> RGVEGSTKSIKYLLFVFNFVFWLAGGVILGVALWLRHDPQTTNLLYLELGDKPAPNTFYVGIYILIAVGAVMMFVGFLGCYGAI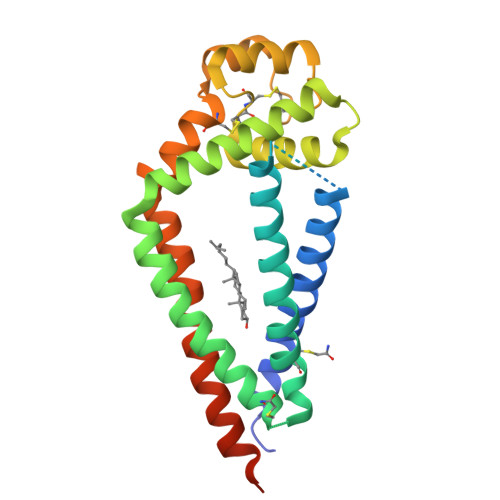QESQCLLGTFFTCLVILFACEVAAGIWGFVNKDQIAKDVKQFYDQALQQAVVDDDANNAKAVVKTFHETLDCCGSSTLTALTTSVLKNNLCPSGSNIISNLFKEDCHQKIDDLFSGKLYLIGIAAIVVAVIMIFEMILSMVLSSGIRNSSVYVPHHHHHHHH> MKLIDKLPSFDRNYIVEEIQGAYDTELNILKEDIDDTFNQLFVDTATWGLDMWEDILCIEKKELDFDTRRSNIKAKMRSRGTSTIEVIKSICEAYTKSETDIKVYSDEFTFVLSFIANN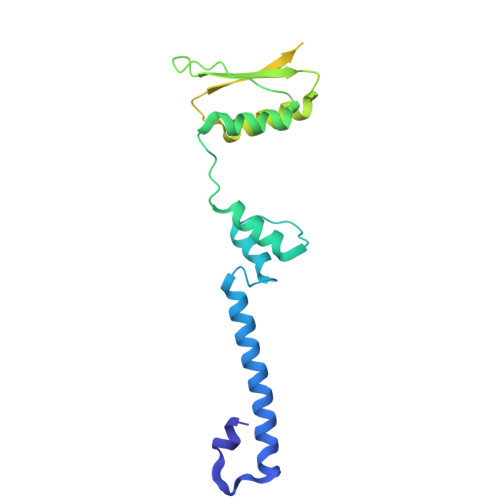CDYKTLLDCSDMIERVKPAHLLHYLEPIILDKSMVYCGGGMVCSEEVKVHPYFEPIIKCSAVVNCGAGMISREEIKVYPLSIKCIENNCKINIAIANDTGVENVVVYPKSEVV N''-(4-(5-((1H-BENZIMIDAZOL-2-YLAMINO)METHYL)-2-THIENYL)-1,3-THIAZOL-2-YL)GUANIDINE 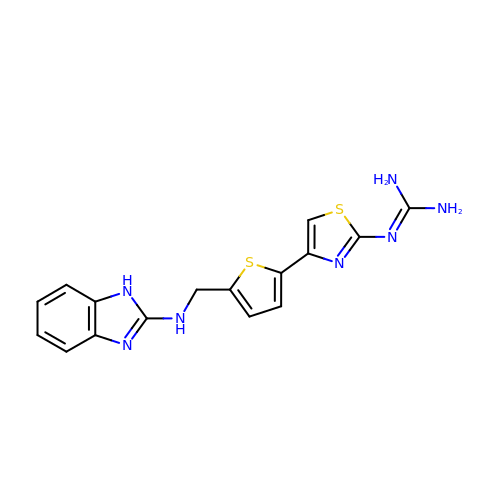| C16 H15 N7 S2 | CKJGKHXCUDWFDC-UHFFFAOYSA-N>[2x]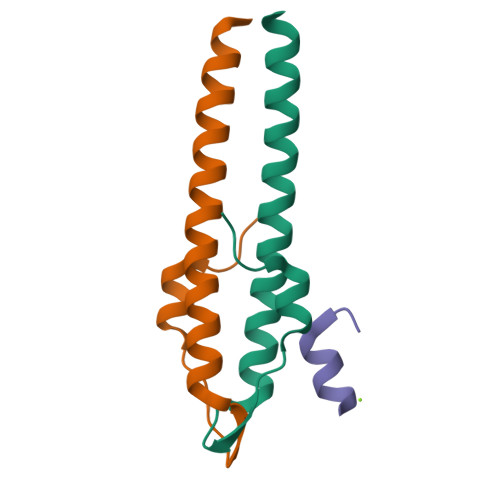GHMKVKLSAKEILEKEFKTGVRGYKQEDVDKFLDMIIKDYETFHQEIEELQQENLQLKKQLEE;> MSDQFNSREARRKANSK>MCGRFLRRLLAEESRRSTPVGRLLLPVLLGFRLVLLAASGPGVYGDEQSEFVCHTQQPGCKAACFDAFHPLSPLRFWVFQVILVAVPSALYMGFTLYHVIWHWELSGKGKEEETLIQGREGNTDVPGAGSLRLLWAYVAQLGARLVLEGAALGLQYHLYGFQMPSSFACRREPCLGSITCNLSRPSEKTIFLKTMFGVSGFCLLFTFLELVLLGLGRWWRTWKHKSSSSKYFLTSESTRRHKKATDSLPVVETKEQFQEAVPGRSLAQEKQRPVGPRDA[6x]

Connexin family proteins assemble into hexameric channels called hemichannels/connexons, which function as transmembrane channels or dock together to form gap junction intercellular channels (GJIChs). Human Cx31.3/GJC3, which is expressed in oligodendrocytes of the central nervous systems, does not form intercellular channels. We determined the cryo–electron microscopy structures of human connexin 31.3 (Cx31.3)/GJC3 hemichannels in the presence and absence of calcium ions and with a hearing-loss mutation R15G at 2.3-, 2.5-, and 2.6-Å resolutions, respectively. We also found that the hemichannel has a pore with a diameter of ~8 Å and selectively transports chloride ions.

While the overall structure did not change with Ca2+ ions, we found small but substantial changes in map densities in a deep tunnel at the interprotomer interface around the acidic band. In the structure with Ca2+ ions, although we could not distinguish Ca2+ densities from water densities due to large overlaps of Ca2+ and water positions, we could observe substantial changes in map densities in and around the Ca2+-binding tunnel. First, the density blobs corresponding to W1 to W4 are considerably smeared, indicating that the water-mediated interaction network is disturbed by Ca2+ ions. In the hemichannel structure with Ca2+ ions, we have not observed close coordination by more than one residue but found many putative binding sites, especially in the Ca2+-binding tunnel. This suggests that Ca2+ ions may play its inhibitory role via multiple weak interactions with functionally important acidic residues, including E47, D66, and E187. Although Ca2+ ions may not strongly bind to E47 and E187 in the tunnel, the dynamic interaction between these residues and Ca2+ ions in the tunnel could disturb the interprotomer interactions, including water-mediated ionic interaction between E47 and R184 and the salt bridge between E187 and R75. In addition, the interaction of D66 with R171 appeared to be weakened by Ca2 binding. The Cx31.3 hemichannel structure in the presence of Ca2+ ions also showed no conformational change, except for several side-chain conformations, compared with its Ca2+-free structure. This suggests that the permeant selectivity could be changed by extracellular Ca2+ ions through the positive electrostatic barrier mechanism, which is proposed on the basis of the Ca2+-bound Cx26 GJICh structure. Ca2+ binding seems to be not strong enough to drive a large conformational change of hemichannel or GJICh at least in detergent environments, and an additional factor, possibly lipids, may be required for the complete channel closing by Ca2+ binding.> GGGMMAKIIVKKSNPLKGSVKIDGAKNAVLPIIAATLLANGKSTLNGVPNLRDVHVISDLLRHVGAEVEYKENTLTVDASNIKTCEAPYELVRKMRASFLVMGPLLARFNSTKISMPGGSAIGTRPIDLHLKGFKALGAKIE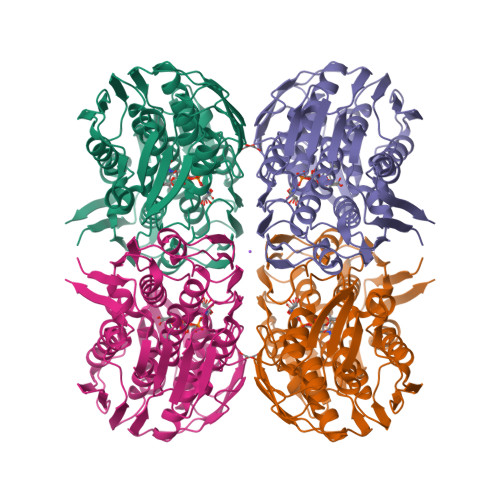MDHGFVEAATEKLVGNKLYLDFPSVGATENIMMAASLAEGTTIIENAAEEPEIVDLANFLNEMGADVKGAGTNTIKIKGVKELKGAEHNVIPDRIEAATYMVAAAMTKGDITVENVLMEHLKPVVAKLREAGCEITEMDNSVRVVGPKVLKPIDIKTLPHPGFPTDVQAQFMAMLTVANGTGVVIETVFENRFMHVAEFNRMGANIKIDGRSAVVNGVDELHGAAVNATDLRAGAALILCGLIAEGETQIGEIYHIQRGYVDIDKKITALGGQIEIVED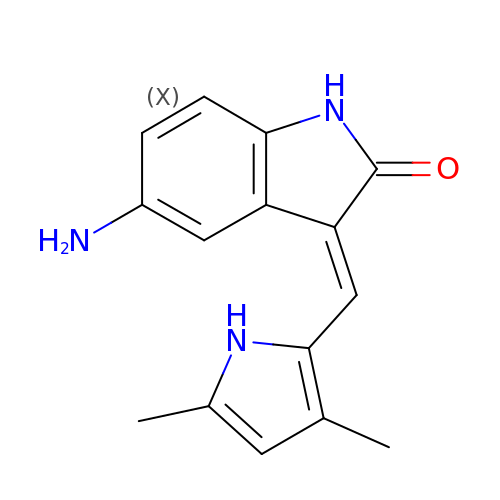(3Z)-5-amino-3-[(3,5-dimethyl-1H-pyrrol-2-yl)methylidene]-1,3-dihydro-2H-indol-2-one | C15 H15 N3 O | XYONNOXYJMPBMA-GHXNOFRVSA-N3-C-carboxy-2-deoxy-D-erythro-pentaric acid | C6 H8 O8 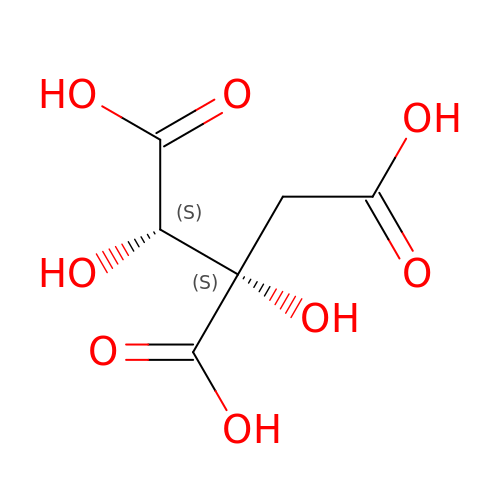| ZMJBYMUCKBYSCP-CVYQJGLWSA-N>MNHKHHHHHHSSGLVPRGSAMGFDDKILLITGGTGSFGNAVMKRFLDSNIKEIRIFSRDEKKQDDIRKKYNNSKLKFYIGDVRDSQSVETAMRDVDYVFHAAALKQVPSCEFFPVEAVKTNIIGTENVLQSAIHQNVKKVICLSTDKAAYPINAMGISKAMMEKVFVAKSRNIRSEQTLICGTRYGNVMASRGSVIPLFIDKIKAGEPLTITDPDMTRFLMSLEDAVELVVHAFKHAETGDIMVQKAPSSTVGDL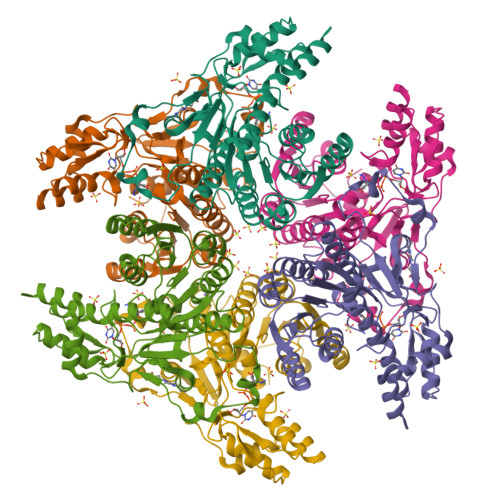ATALLELFEADNAIEIIGTRHGEKKAETLLTREEYAQCEDMGDYFRVPADSRDLNYSNYVETGNEKITQSYEYNSDNTHILTVEEIKEKLLTLEYVRNELNDYKASMR[2x]>[2x]GAMGSGGGGEHQH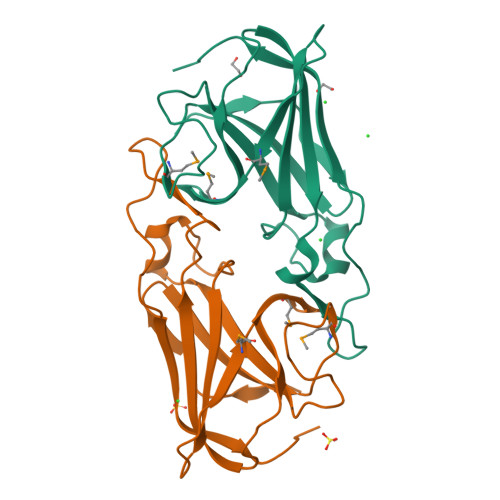GEEMMAAVPAPDAEGAAGFDEFPIGEDRDVGPLHVGGVYFQPVEMHPAPGAQPSKEEADCHIEADIHANEAGKDLGYGVGDFVPYLRVVAFLQKHGSEKVQKVMFAPMNAGDGPHYGANVKFEEGLGTYKVRFEIAAPSHDEYSLHIDEQTGVSGRFWSEPLVAEWDDFEWKGPQW> MGFIGNSLPMQAVYRVIESAASSKATVFITGESGTGKEVCAEAIHAASPRHDKPFIALNCAAIPKDLIESELFGHVKGAFTGASTERQGAVEMAHNGTLMLDELCEMDLDLQSKLLRFIQTGTYQKVGSSKMSSVDVRFVCATNRNPWEEVQEGRFREDLYYRLHVIPISLPPLRERGGDIIEIAHALLGLMSLEEGKSFSRFSEPVLRLFESYSWPGNVRELQNVIRNIVVLNTDDEVKLEMVPPPILEHHH

Here, we use X-ray crystallography to study LuxO, the central quorum sensing regulator in Vibrio cholerae and related bacteria. LuxO belongs to the subfamily of AAA+ ATPases known as bacterial enhancer-binding proteins (bEBPs). In LuxO, as in NtrC proteins, the phosphorylation of an aspartate located within the R-domain activates the C domain for ATP hydrolysis and the opening/activation of σ54-dependent promoters. Here, we present crystal structures and in vitro and in vivo functional studies of LuxO that together reveal what is, to our knowledge, an entirely novel mechanism of AAA+ protein regulation, in which a regulatory segment of the protein prevents substrate ATP binding and hydrolysis by occupying a portion of the enzyme active site.

To characterize the mechanism of AzaU inhibition of LuxO, we crystallized V. angustum LuxO-C in the absence of ligands (apo), in the presence of ATP, and in the presence of AzaU. All three protein structures are highly similar (rms deviation < 0.5 Å). Rather than forming closed rings, V. angustum LuxO monomers in the crystals form continuous helical arrays with six subunits per turn. We also observed the same helical arrays of LuxO monomers in crystal structures of the V. angustum C domain alone (LuxO-C), either as the apo-protein, with ATP bound, or with the inhibitor AzaU bound (discussed below). Indeed, the monomer–monomer interfaces observed in our LuxO-RC and LuxO-C structures are similar to those observed in NtrC1 and other AAA+ proteins that crystallize in closed-ring arrangements.(2R,3R,4S)-2-(hydroxymethyl)-1-(quinolin-8-ylmethyl)pyrrolidine-3,4-diol 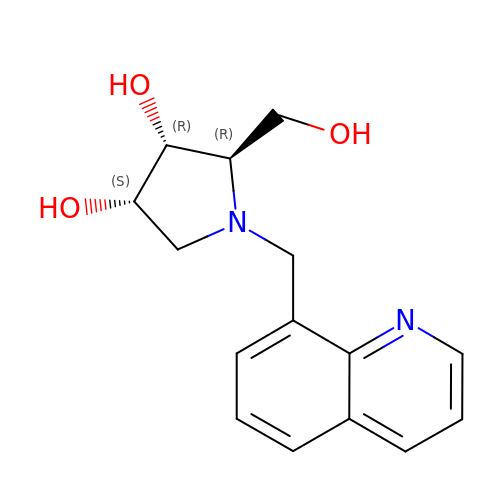| C15 H18 N2 O3 | MZDAWIBFZPTLPG-VNHYZAJKSA-N>SAAATQAVPAPNQQPEVFCNQIFINNEWHDAVSRKTFPTVNPSTGEVICQVAEGDKEDVDKAVKAARAAFQLGSPWRRMDASHRGRLLNRLADLIERDRTYLAALETLDNGKPYVISYLVDLDMVLKCLRYYAGWADKYHGKTIPIDGDFFSYTRHEPVGVCGQIIPWNFPLLMQAWKLGPALATGNVVVMKVAEQTPLTALYVANLIKEAGFPPGVVNIVPGFGPTAGAAIASHEDVDKVAFTGSTEIGRVIQVAAGSSNLKRVTLELGGKSPNIIMSDADMDWAVEQAHFALFFNQGQCCCAGSRTFVQEDIYDEFVERSVARAKSRVVGNPFDSKTEQGPQVDETQFKKILGYINTGKQEGAKLLCGG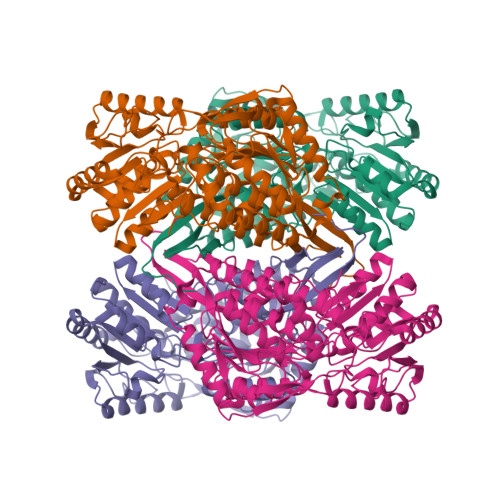GIAADRGYFIQPTVFGDVQDGMTIAKEEIFGPVMQILKFKTIEEVVGRANNSTYGLAAAVFTKDLDKANYLSQALQAGTVWVNCYDVFGAQSPFGGYKMSGSGQELGEYGLQAYTEVKTVTVKVPQKNS[8x]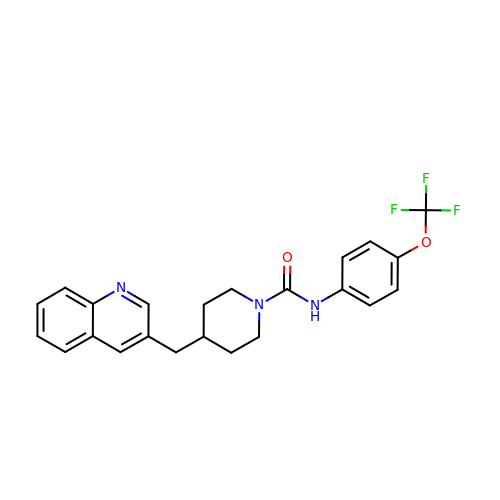4-[(quinolin-3-yl)methyl]-N-[4-(trifluoromethoxy)phenyl]piperidine-1-carboxamide | C23 H22 F3 N3 O2 | QEMFEXNNXOLBRG-UHFFFAOYSA-N>RSDSPEIPFQAAAGPSDGLDASSPGNSFVGLRVVAKWSSNGYFYSGKITRDVGAGKYKLLFDDGYECDVLGKDILLCDPIPLDTEVTALSEDEYFSAGVVKGHRKESGELYYSIEKEGQRKWYKRMAVILSLEQGNRLREQYGLGPYEAVTPLTKAADISL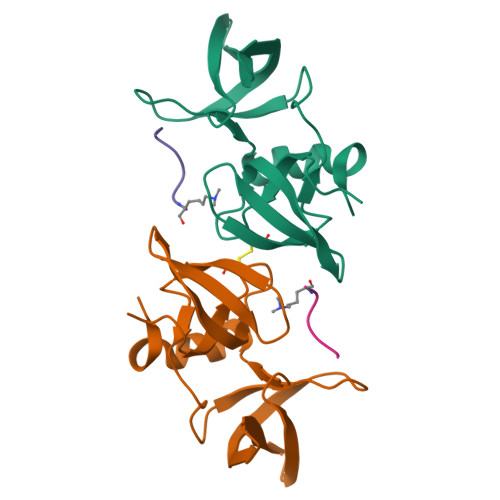DNLVEGKRKRRSNVS[2x];>[2x]GNIYISPLKSPYKISEC> MGHHHHHHHHHHSSGHIDDDDKHMAGGAAQESKSFAVGMFKGQLTTDQVFPYPSVLNEEQTQFLKELVEPVSRFFEEVNDPAKNDALEMVEETTWQGLKELGAFGLQVPSELGGVGLCNTQYARLVEIVGMHDLGVGITLGAHQSIGFKGILLFGT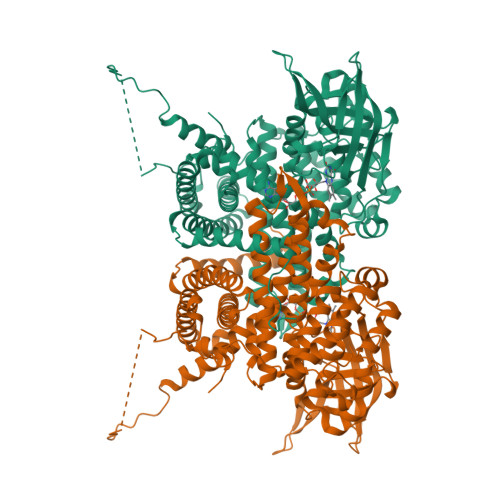KAQKEKYLPKLASGETVAAFCLTEPSSGSDAASIRTSAVPSPCGKYYTLNGSKLWISNGGLADIFTVFAKTPVTDPATGAVKEKITAFVVERGFGGITHGPPEKKMGIKASNTAEVFFDGVRVPSENVLGEVGSGFKVAMHILNNGRFGMAAALAGTMRGIIAKAVDHATNRTQFGEKIHNFGLIQEKLARMVMLQYVTESMAYMVSANMDQGATDFQIEAAISKIFGSEAAWKVTDECIQIMGGMGFMKEPGVERVLRDLRIFRIFEGTNDILRLFVALQGCMDKGKELSGLGSALKNPFGNAGLLLGEAGKQLRRRAGLGSGLSLSGLVHPELSRSGELAVRALEQFATVVEAKLIKHKKGIVNEQFLLQRLADGAIDLYAMVVVLSRASRSLSEGHPTAQHEKMLCDTWCIEAAARIREGMAALQSDPWQQELYRNFKSISKALVERGGVVTSNPLGF The tripartite motif (TRIM) consists of an N-terminal RING domain, one or two B-box domains and a C-terminal coiled-coil domain. Almost 50% of all TRIM proteins - including TRIM20 - carry a B30.2 domain immediately after the coiled-coil domain of the central TRIM motif. TRIM20 is associated with the auto-inflammatory disease Familial Mediterranean Fever (FMF) and it is involved in the modulation of the pro-inflammatory cytokine pro-interleukin-1β (pro-IL-1β)67. TRIM20 is considered to inhibit the inflammasome mediated maturation of pro-IL-1β8, but it can also potently induce the maturation of this cytokine.

Here we present the crystal structure of the TRIM20 coiled-coil/B30.2 fragment at 2.4 Å resolution. TRIM20Δ413 crystallized in space group P21 with 6 chains in the asymmetric unit. In the crystal TRIM20Δ413 forms a clear dimer with a coat-hanger-like shape. Dimerization is achieved by the coiled-coil motifs (E414–N586) that form an elongated and slightly bend scaffold for the globular B30.2 domain (E589–G776). The B30.2 domain is connected to the scaffold domain by a flexible loop (V587-P588) that acts as a hinge. The subunits of the TRIM20Δ413 dimer arrange in an antiparallel fashion along helix α1 with a shared interface of more than 4700 Å2. As a result, the presumed B-box domains at the N-termini of TRIM20Δ413 are positioned approximately 170 Å apart from each other, whereas the B30.2 domains are close to the 2-fold axis of the dimer. Within the TRIM20Δ413 dimer the B30.2 domains neither interact with each other nor with the CHS domain, supporting the assumption that the orientation of the B30.2 domain might be highly flexible in solution. However, B30.2 and CHS domains share interfaces between neighboring dimers. These inter-molecular interfaces cover areas between 1710 and 1950 Å2 and are formed by the extended proline-rich stretch of the CHS domain that runs through a shallow surface cleft between the Pry- and Spry segments of the neighboring B30.2 domain. Therefore, we refer to the conformation seen in the crystal structure of TRIM20Δ413 as the closed state.

>[6x]XSEVALEHKKKIQKQLEHLKKLRKSGEEQRSYGEEKAVSFLKQTEALKQRVQRKLEQVYYFLEQQEHFFVASLEDVGQMVGQIRKAYDTRVSQDIALLDALIGELEAKECQSEWELLQDIGDILHRAKTVPVPEKWTTPQEIKQKIQLLHQKSEFVEKSTKYFSETLRSEMEMFNVPELIGAQAHAVNVILDAETAYPNLIFSDDLKSVRLGNKWERLPDGPQRFDSCIIVLGSPSFLSGRRYWEVEVGDKTAWILGACKTSISRKGNMTLSPENGYWVVIMMKENEYQASSVPPTRLLIKEPPKRVGIFVDYRVGSISFYNVTARSHIYTFASCSFSGPLQPIFSPGTRDGGKNTAPLTICPVGGQGPDALEVLFQ Here we report the discovery of a new family of DUBs, which we have named MINDY (motif interacting with Ub-containing novel DUB family). Found in all eukaryotes, MINDY-family DUBs are highly selective at cleaving K48-linked polyUb, a signal that targets proteins for degradation. Our structural analyses reveal that the catalytic domain of FAM63A is a distinct folding variant of the superfamily of cysteine proteases. Collectively, our analysis of human MINDY-1 reveals that it is a chain-trimming enzyme, which uses the Ub-binding MIU together with the catalytic domain to cleave K48-linked polyUb chains from the distal end in a stepwise manner.

In order to determine the mechanism of this newly identified DUB, we crystallized the minimal catalytic domain of FAM63A/MINDY-1 spanning residues 110–384 (MINDY-1cat). The structure of MINDY-1cat domain was determined at 3 Å resolution by X-ray crystallography. The asymmetric unit (ASU) contains one molecule of MINDY-1cat with discernible electron density for residues 110–370. The catalytic core domain of MINDY-1 with a dimension of 32 × 64 × 36 Å resembles a light bulb consisting of two subdomains, a central “bulb” subdomain that sits on a “stalk” subdomain, which resembles the base of the bulb. The core of the central bulb subdomain contains a seven-stranded β sheet (β4–β10), where β7 is connected to β8 by a short 310-helix. The stalk subdomain, made up of three α helices (α5–α7), forms a long helical arm that protrudes away from the central domain. We predict the conserved C137 at the N terminus of helix α1 and H319 on the adjacent β6 to be the catalytic residues and these are present in a C-H architecture typical of papain-like peptidases. The third catalytic residue, which serves to polarize the catalytic His, is not obvious in the observed crystal structure. However, in the structure of isolated MINDY-1cat, the active site is in an unproductive conformation and C137 is rotated out of hydrogen bond distance from the other catalytic residues. Therefore, the observed structure is MINDY-1 in an inhibited state.

> GPLGSPEFPGRLEMEPDFYCVKWIPWKGEQTPIITQSTNGPCPLLAIMNILFLQWKVKLPPQKEVITSDELMAHLGNCLLSIKPQEKSEGLQLNFQQNVDDAMTVLPKLATGLDVNVRFTGVSDFEYTPECSVFDLLGIPLYHGWLVDPQSPEAVRAVGKLSYNQLVERIITCKHSSDTNLVTEGLIAEQFLETTAAQLTYHGLCELTAAAKEGELSVFFRNNHFSTMTKHKSHLYLLVTDQGFLQEEQVVWESLHNVDGDSCFCDSDFHLSHSLGKGPGAEGGSGSPE> AREGIIGHYIHHNQRVGVLVELNCETDFVARNELFQNLAKDLAMHIAMMNPRYVSAEEIPAEELEKERQIYIQAA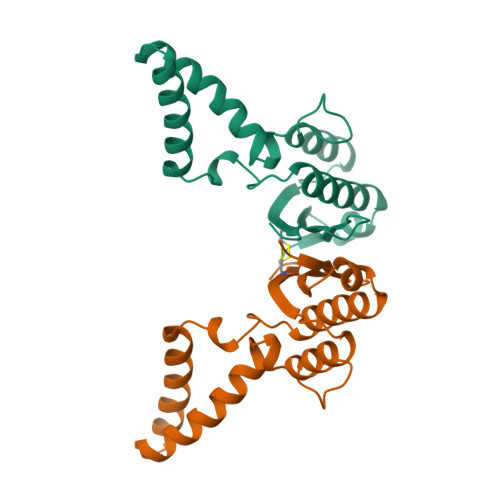LNEGKPQQIAEKIAEGRLKKYLEEVVLLEQPFVKDDKVKVKELIQQAIAKIGENIVVRRFCRFELGAMMC>[75x]QDLMASGNTTVKATFGKD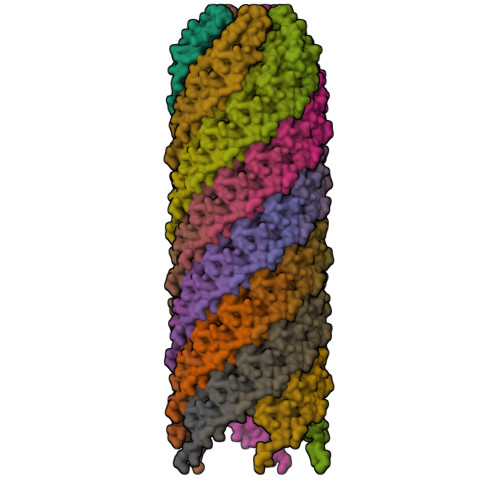SSVVKWVVLAEVLVGAVMYMMTKNVKFLAGFAIISVFIAVGMAVVGL>MHHHHHH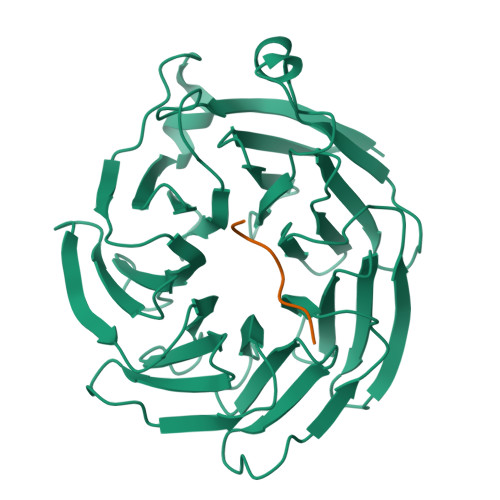HHTFTRYSRLRVIAEIRHGDIFHSANIVSSIEFDRDDELFATAGVSRCIKVFDFSSVVNEPADMQCPIVEMSTRSKLSCLSWNKHEKNHIASSDYEGIVTVWDVTTRQSLMEYEEHEKRAWSVDFSRTEPSMLVSGSDDCKVKVWCTRQEASVINIDMKANICCVKYNPGSSNYIAVGSADHHIHYYDLRNISQPLHVFSGHKKAVSYVKFLSNNELASASTDSTLRLWDVKDNLPVRTFRGHTNEKNFVGLTVNSEYLACGSETNEVYVYHKEITRPVTSHRFGSPDMDDAEEEAGSYFISAVCWKSDSPTMLTANSQGTIKVLVLAA[4x];>[4x]SDQIVPEY>GHMWQENKSWNAHFTEHKSQGVVVLWNENKQQGFTNNLKRANQAFLPASTFKIPNSLIALDLGVVKDEHQVFKWDGQTRDIATWNRDHNLITAMKYSVVPVYQEFARQIGEARMSKMLHAFDYGNEDISGNVDSFWLDGGIRISATE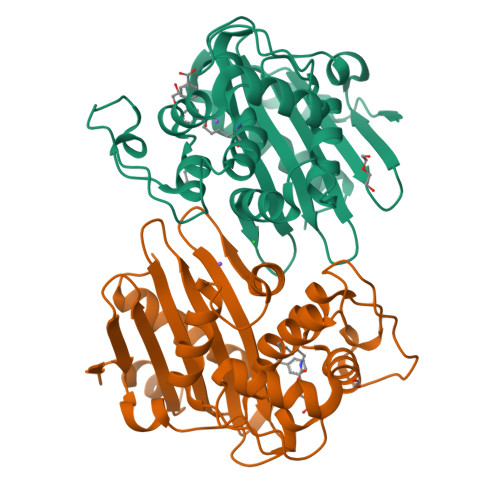QISFLRKLYHNKLHVSERSQRIVKQAMLTEANGDYIIRAKTGYSTRIEPKIGWWVGWVELDDNVWFFAMNMDMPTSDGLGLRQAITKEVLKQEKIIP[4x]>DESQVPDQPSSLHVRPQTNCIIMSWTPPLNPNIVVRGYIIGYGVGSPYAETVRVDSKQRYYSIERLESSSHYVISLKAFNNAGEGVPLYESATTRGSGGSGGSGGSGGSGGSGGSG[2x];>[2x]GMLPPVGVQAVALTHDAVRVSWADNSVPKNQKTSEVRLYTVRWRTSFSASAKYKSEDTTSLSYTATGLKPNTMYEFSVMVTKNRRSSTWSMTAHATTYEAAPTSAPKDLTVITREGKPRAVIVSWQPPLEANGKITAYILFYTLDKNIPIDDWIMETISGDRLTHQIMDLNLDTMYYFRIQARNSKGVGPLSDPILFRTLKLEVL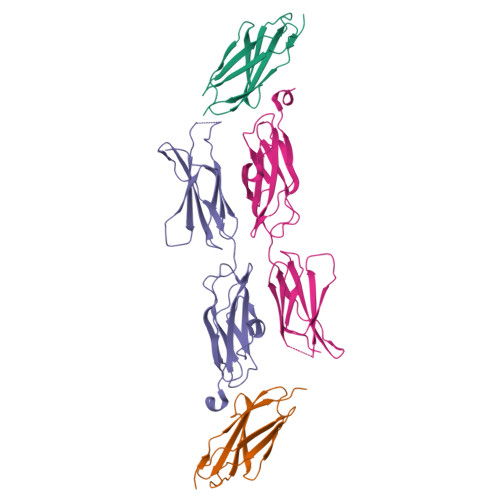FQ>[6x]MNHKVHHHHHHIEGRHMAVVKEVLEIAEKIKNMEIR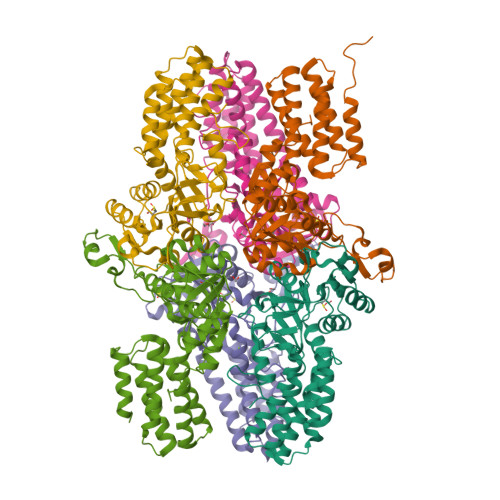GAGKIARSAAYALQLQAEKSKATNVDEFWKEMKQAAKILFETRPTAVSLPNALRYVMHRGKIAYSSGADLEQLRFVIINAAKEFIHNSEKALERIGEFGAKRIEDGDVIMTHCHSKAAISVMKTAWEQGKDIKVIVTETRPKWQGKITAKELASYGIPVIYVVDSAARHYMKMTDKVVMGADSITVNGAVINKIGTALIALTAKEHRVWTMIAAETYKFHPETMLGQLVEIEMRDPTEVIPEDELKTWPKNIEVWNPAFDVTPPEYVDVIITERGIIPPYAAIDILREEFGWALKYTEPWED> SMGNLIKVLTRDIDHNASHFFLDFENAQPTEAEREIFNQVNVVLKDAEGILNDLQSYRGAGHEIREAIQHPNDENLQEKAWSAVCPLVGKLKKFYEFSQRLEAALHGLLGALTSTPYSPTQHLEREQALAKQFAEILHFTLRFDELKMTNPAIQNDFSYYRRTLSRMRINNVPAEGENEVNNELANRMSLFYAEATPMLKTLSDATTKFVSDNKSLPIENTTDCLSTMASVCRVMLETPEYRSRFASEETVSFCLRVMVGVIILYDHVHPVGAFAKTSKIDMKGCIKVLKDQPPNSVEGLLNALRYTTKHLNDETTSKQIKTMLQ

Previously known as FAM49B, CYRI-B is a protein that is highly conserved across the Eukaryota and has recently been revealed to be a key regulator of Rac1 activity. CYRI-B binding has been reported to block various Rac1-dependent signalling cascades in the cell, thereby controlling multiple critical cellular functions including T-cell activation, membrane protrusion, chemotaxis and cell migration. Our structure, the first to be reported of any member of the CYRI family, reveals a protein that is entirely composed of α-helices and organized into three distinct subdomains. The similarity in structure suggests that CYRI-B interacts with Rac1 in the same manner as CYFIP1 and therefore regulates actin-dependent processes by competition with the WRC for Rac1 binding.

We therefore produced SeMet-substituted protein, which allowed us to determine the structure of CYRI-B by SAD phasing. Solved by X-ray crystallography at 2.4 Å resolution using the SAD method, the structure reveals three distinct, entirely α-helical, subdomains and high structural similarity to a conserved domain of CYFIP1. The native and SeMet-derivatized protein crystals have similar unit-cell dimensions and belong to the same ortho­rhombic space group, P212121. They were solved at resolutions of 2.37 and 2.40 Å, respectively. In both cases, a single molecule is present in the asymmetric unit. The two models are nearly identical and could be aligned with a Cα r.m.s.d. of 0.29 Å for 320 atoms. In both the native and the SeMet-derivatized structures, the flexible loop composed of residues 171–175 was too disordered to build and is therefore missing from the final models. This loop connects helices α7 and α8 of the medial subdomain. Biochemical analyses of R. typus CYRI-B were conducted to confirm the oligomeric state of the protein found by X-ray crystallography. As presented in Fig. 2(a), the native and SeMet-derivative proteins migrate as a single band on both native and SDS–PAGE gels. The gel electrophoresis and SEC results corroborate the crystallographic data, confirming the monomeric state of CYRI-B in solution.> LGLDCDEHSSESRCCRYPLTVDFEAFGWDWIIAPKRYKANYCSGQCEYMFMQKYPHTHLVQ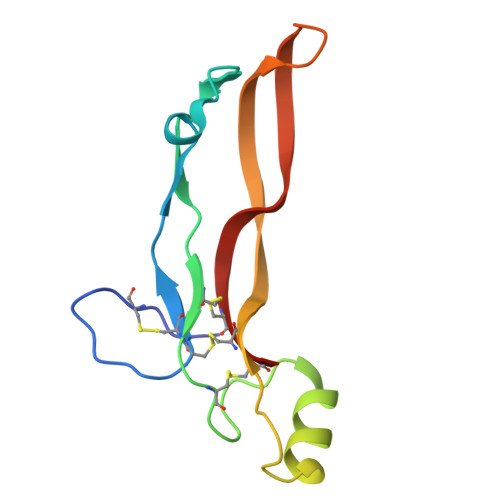QANPRGSAGPCCTPTKMSPINMLYFNDKQQIIYGKIPGMVVDRCGCS> MNNNKAEADTSSSMADPETRPTYTTHHLAIPSGVTQDEFDELKQSVVEFHTYQLSQNQCSSLLAQRIRAPNDVVWSIVRRFDQPQTYKHFIKSCSVSDNFTMAVGSTRDVNVISGLPAATSTERLDILDDDRQVTGFSIIGGEHRLRNYRSVTSVHGFNRDGAICTVVLESYVVDVPEGNTEEDTRLFADTVVKLNLQKLVSVAESQVI;> RSVYELDCIPLWGTVSIQGNRSEMEDAFAVSPHFLKLPIKMLMGDHEGMSPSLTHLTGHFFGVYDGHGGHKVADYCRDRLHFALAEEIERIKDELCKRNTGEGRQVQWDKVFTSCFLTVDGEIEGKIGRAVVGSSDKVLEAVASETVGSTAVVALVCSSH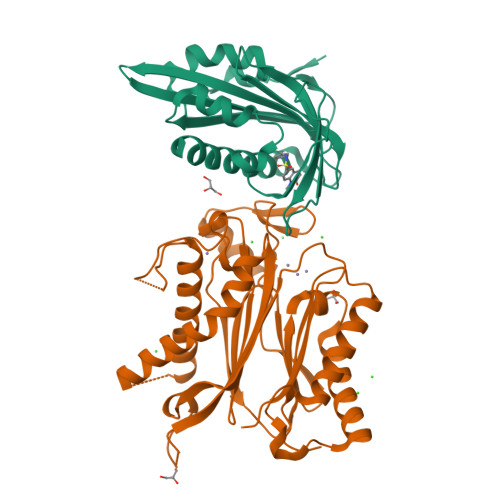IVVSNCGDSRAVLFRGKEAMPLSVDHKPDREDEYARIENAGGKVIQWQGARVFGVLAMSRSIGDRYLKPYVIPEPEVTFMPRSREDECLILASDGLWDVMNNQEVCEIARRRILMWHKKNGAPPLAERGKGIDPACQAAADYLSMLALQKGSKDNISIIVIDLKAQR> APAAVDWRARGAVTAVKDQGQCGSCWAFSAIGNVECQWFLAGHPLTNLSEQMLVSCDKTDSGCSGGLMNNAFEWIVQENNGAVYTEDSYPYASG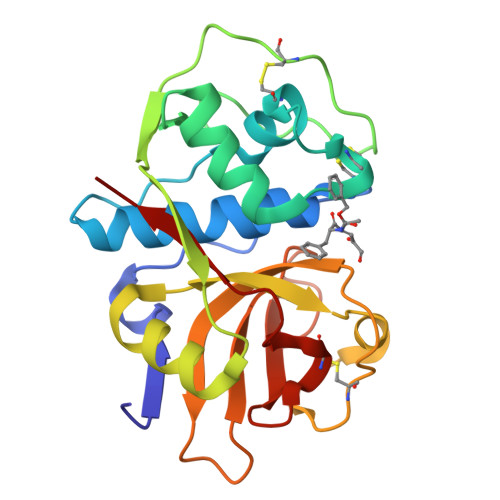EGISPPCTTSGHTVGATITGHVELPQDEAQIAAWLAVNGPVAVAVDASSWMTYTGGVMTSCVSEQLDHGVLLVGYNDSAAVPYWIIKNSWTTQWGEEGYIRIAKGSNQCLVKEEASSAVVG>GGGGCCCC[2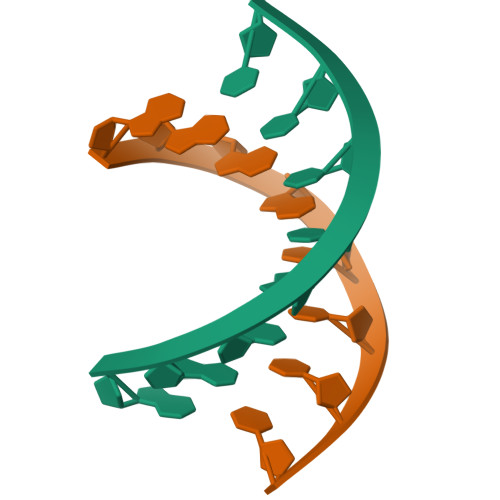x]>[2x]MNSDIPFDLIQERTGVPS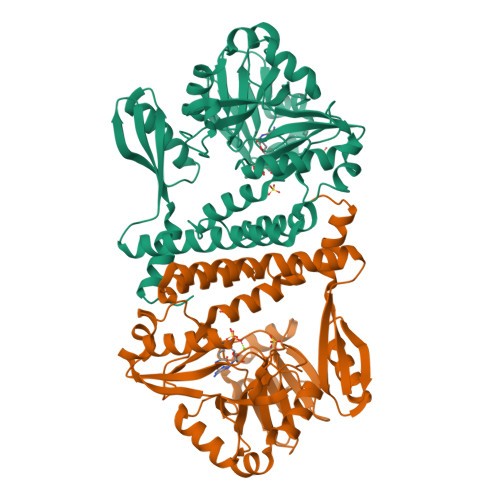SRLKVAFARGSLRLLESAGMQALLFKKPLGDLEAGTVIYLGDETEVIRGFPKIRRTLLLSPTIQEHFRDRVAVEEKMNGYNVRIACLSSGETVALTRGGHVCPFTTRKAQELLDLSEFFREHPDLVICGEMIGRDNPYVSQDYPEVGPLGFRVFDLREKNTNRPLPVEERRALLDSYGLPNVRLFGVYPIEEAASEVADIIRALGMAGREGVVMKDPSMEVPPLKYTSSQAHARELAYAFSYPFDFGRPFFFSRVIREGFQAYELDESDDETRERARRLGEAIIYPMLERIKSISAGEAAYEDTVIDVEDREAAEEFIRHLVRLGVSATLADYRDGRATIRRFYQSTTDRINNYLKGGLY(2R,4S)-N^1^-(4-chlorophenyl)-4-(2,4-difluorophenyl)-4-hydroxy-N^2^-(2-oxo-2H-1,3'-bipyridin-6'-yl)pyrrolidine-1,2-dicarboxamide | C28 H22 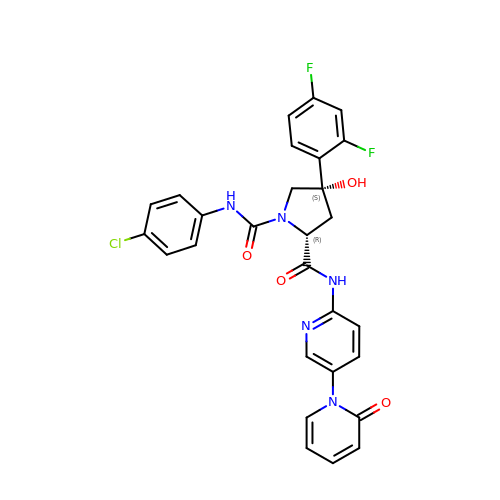Cl F2 N5 O4 | BGECSWGTDIXGJY-QDPGVEIFSA-N>[7x]DNYIYSTEVGGVGGTPFTFMQESGTITSIKFNWSDQYKLLHHIEVKFINNANIYATGDPKGNHEVILEIDDDETIIGSVIGYKKGNDGRCT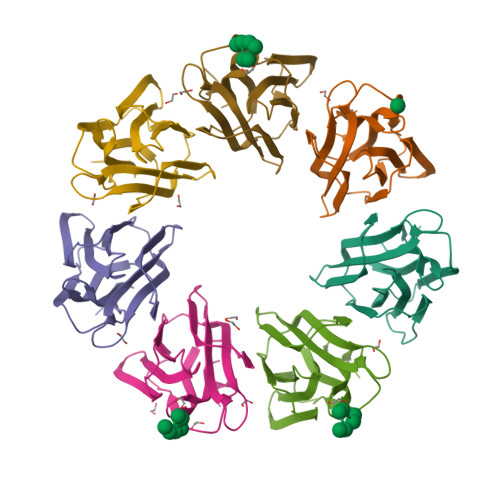GVKLTTSKGKSIMAGYFEESLITTYTGKLAGIKGGAGSDIDRLGLIFLK The ReAV enzyme from Rhizobium etli, a representative of Class 3 L-asparaginases, is sequentially and structurally different from other known L-asparaginases. Asparaginases (EC 3.5.1.1) catalyze the hydrolysis of L-asparagine, generating L-aspartate and ammonia. ReAV is a homodimeric protein, with each subunit containing a highly specific zinc-binding site created by two cysteines, a lysine, and a water molecule. Two Ser-Lys tandems (Ser48-Lys51, Ser80-Lys263) are located in the close proximity of the metal binding site, with Ser48 hypothesized to be the catalytic nucleophile.

The absence of Lys263 led to only subtle structural rearrangements and atomic shifts within the active site, largely consistent in the four protein chains. A water molecule fills the available space left by the lysine side chain, marking the site of its Nζ atom and maintaining the original pattern of hydrogen bonds. The Lys263 mutation affected the conformational state and hydration pattern of Ser48. The major rotamer of Ser48, with a refined occupancy of 0.7, can no longer form H-bonds with the Oγ atom of Ser80 and the Nζ atom of Lys51. Instead, it interacts with the carbonyl oxygen atom of Leu264 and two water molecules, mimicking the arrangement of two water molecules in the typical triangular configuration, though with increased O…O distances (2.70–2.90 Å). The zinc cation nearly fully occupies the metal binding site, with a refined occupancy of 0.8, shared with the coordinated water molecule. As observed in the previously described mutant structures, a sulfate ion (derived from the crystallization solution and present at 0.7 occupancy) is bound near the zinc cation, forming H-bonds with the main-chain N atoms of Gly188 and Cys189, the Nη atom of Arg47, and several water molecules, one of which is part of the metal coordination sphere. As observed in the S80A mutant structure, the side chain of Cys249 exhibits a chemical modification, modeled as S-hydroxycysteine. In the K263A mutant structure, the major rotamer of Ser48 shifts in response to the mutation, moving away from Lys51. This leads to stereochemistry that is suboptimal for the nucleophilic attack and prevents activation by the basic Lys51 side chain.

>[4x]GIDPFTMTPSEDFVVTDRGGIVENSHRVHAAVVDAKGRLLYALGNPTRMTLARSAAKPAQALAILETEGVAGYGFDDADIALMCASHSSEDRHIARTRAMLSKIKAEEADLRCGGHPSLSEMVNRSWIKQDFIPTAVCSNCSGKHVGMLAGARAIGAGTDGYHLPDHPMQGRVKRTVAELCDLDAGDVEWGTDGCNLPTPAFPLDRLGRIYAKLASAADGSDAGEGQSTRCAALAHIFRAMARHPEMVAGEGRYCTMLMRAFDGALVGALGADASYAIGVRASDATRQLGTDGALGISVKIEDGNLEMLYAVVTELLERLGIGSPDVRSQLASFHHPQRVNTMGVTTGGVSFPFKLRGSKSNVDDPRLAAVAR>MDPLTVYKNSVKQQIDSADLLVANLVNENFVLSEKLDTKATEIKQLQKQIDSLNAQVKELKTQTSQQAENSEVIKDLYEYLCNVRVHKSYEDDSGLWFDISQGTH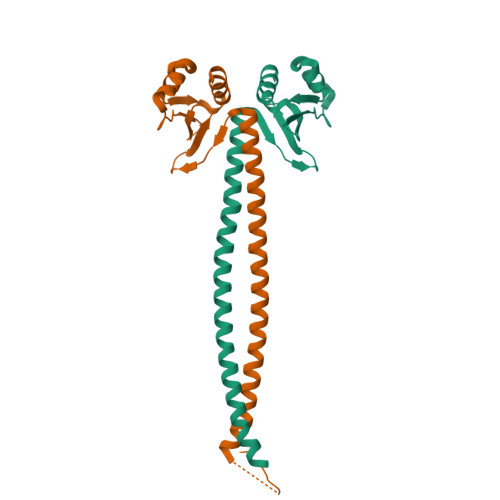SGGSSDDYSIMDYKLGFVKGQAQVTEVIYAPVLKQRSTEELYSLQSKLPEYLFETLSFPLSSLNQFYNKIAKSLNKKREKKDETE[4x]> GPHMGLVQRC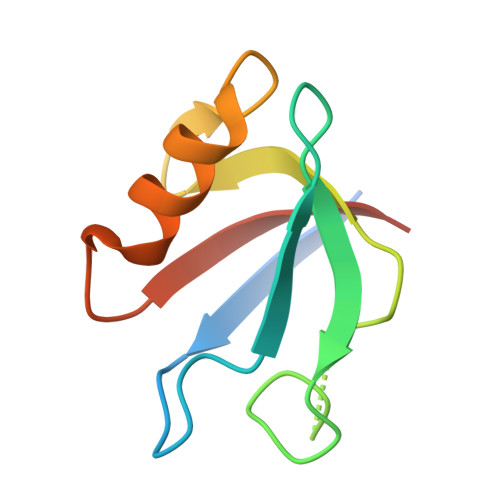VIIQKDQHGFGFTVSGDRIVLVQSVRPGGAAMKAGVKEGDRIIKVNGTMVTNSSHLEVVKLIKSGAYVALTLLGSSPS> MILAKTKSGKTIDLTFAHEVVKSNVKNVKDRKGKEKQVLFNGLTTSKLRNLMEQVNRLYTIAFNSNEDQLNEEFIDELEYLKIKFYYEAGREK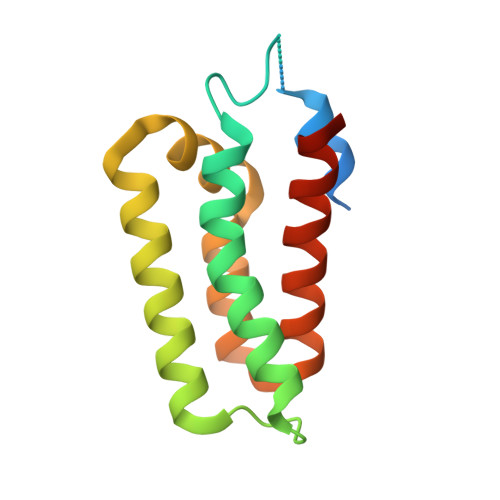SVDEFLKKTLMFPIIDRVIKKESKKFFLDYCKYFEALVAYAKYYQKED>MSLIDPRAIIDPSARLAADVQVGPWSIVGAEVEIGEGTVIGPHVVLKGPTKIGKHNRIYQFSSVGEDTPDLKYKGEPTRLVIGDHNVIREGVTIHRGTVQDRAETTIGDHNLIMAYAHIGHDSVIGNHCILVNNTALAGHVHVDDWAILSGYTLVHQYCRIGAHSFSGMGSAIGKDVPAYVTVFGNPAEARSMNFEGMRRRGFSSEAIHALRRAYKVVYRQGHTVEEALAELAESAAQFPEVAVFRDSIQSATRGITR[6x]

LpxA and LpxD are functionally and structurally similar, sharing a homotrimer architecture and conserved active site features, especially in the acyl-chain binding pockets that reside in the dimer interface of the β-helix trimer core. Herein we report the discovery of several small molecules that bind to both P. aeruginosa LpxA and LpxD with μM affinity, identified using a targeted structure-based methodology that utilizes molecular docking, surface plasmon resonance (SPR) bioanalysis, and high-resolution X-ray crystallography.

The complex structure of LpxA with compound 2 was solved at 2.00 Å. Corresponding ligand electron density is seen at all 6 active sites within the asymmetric unit. Similar to 1, two binding modes were observed for compound 2, with differences mainly in the conformation of the flexible side chain bearing the carboxyl group. Five out of the six copies of compound 2 adopt a binding conformation represented by pose 1, with the carboxyl group placed near His156. In the other binding mode (pose 2), the carboxyl group is pushed away from His156 due to a new conformation of this residue. Many of the interactions formed by compound 1 with LpxA are also seen with compound 2, especially for pose 1, including the hydrogen bonds between the carboxyl group and Gln157, and between the carbonyl group and Gly151. Meanwhile, the benzoxazine ring forms non-polar contacts with Ala136 and Val132, and the hydrocarbon ruler Met169. Whereas both the ring structures of compounds 1 and 2 are buried in the acyl chain pocket, the benzoxazine ring of compound 2 is pulled slightly outward, likely due to the hydrogen bonding interactions between the substituted amide group and residues His121 and Asp70 that have been proposed to be directly involved in catalysis. The docking result predicted that compound 2 would be buried deeper in the acyl chain pocket, similar to 1. This is likely due to the protein template used in the rigid docking procedure, which failed to account for the HB interactions with His121, Asp70 and Gln157.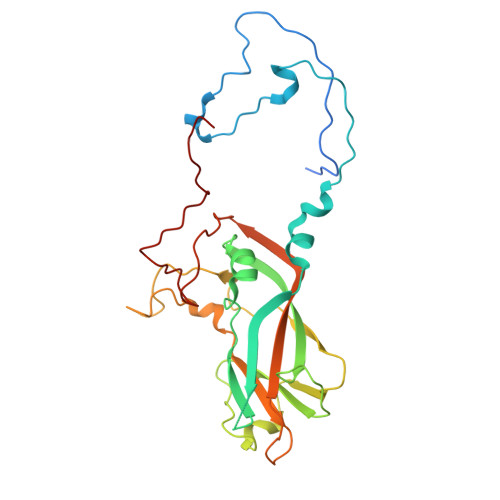> GDPIADMIDQTVNNQVNRSLTALQVLPTAANTEASSHRLGTGVVPALQAAETGASSNASDKNLIETRCVLNHHSTQETAIGNFFSRAGLVSIITMPTTDTQNTDGYVNWDIDLMGYAQLRRKCELFTYMRFDAEFTFVVAKPNGVLVPQLLQYMYVPPGAPKPTSRDSFAWQTATNPSVFVKMTDPPAQVSVPFMSPASAYQWFYDGYPTFGEHLQANDLDYGQCPNNMMGTFSIRTVGTEKSPHSITLRVYMRIKHVRAWIPRPLRNQPYLFKTNPNYKGNDIKCTSTSRDKITTL>MKVRAQVPTVKNATNFNMVADSKTSVGSTLENLKAAIAGETGAHAKYTAFAKAAREQGYEQIARLFEATAAAELIHIGLEYALVAEMEPGYEKPTVAAPSAYSCDLNLISGANGEIYETSDMYPAFIRKAQEEGNSKAVHVFTRAKLAESVHAERYLAAYNDIDAPD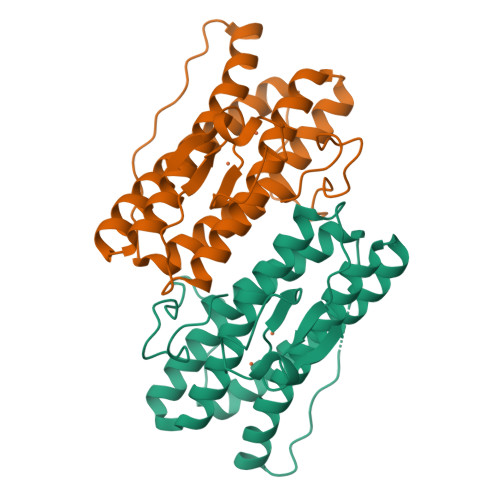DDKFHLCPICGYIHKGEDFEKCPICFRPKDTFTAY[2x]>MTLGRRLACLFLACVLPALLLGGTALASEIVGGRRARPHAWPFMVSLQLRGGHFCGATLIAPNFVMSAAHCVANVNVRAVRVVLGAHNLSRREPTRQVFAVQRIFENGYDPVNLLNDIVILQLNGSATINANVQVAQLPAQGRRLGNGVQCLAMGWGLLGRNRGIASVLQELNVTVVTSLCRRSNVCTLVRGRQAGVCFGDSGSPL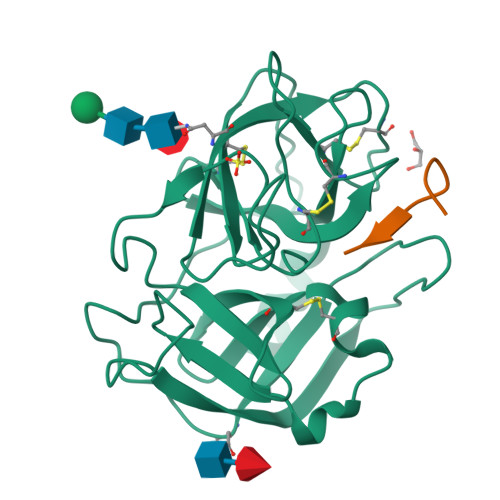VCNGLIHGIASFVRGGCASGLYPDAFAPVAQFVNWIDSIIQRSEDNPCPHPRDPDPASRTH[4x];>VSSPVSTM[4x]>MSTTANKERCLEMVAAWNRWDVSGVVAHWAPDVVHYDDEDKPVSAEEVVRRMNSAVEAFPDLRLDVRSIVGEGDRVMLRITCSATHQGVFMGIAPTGRKVRWTYLEELRFSEAGKVVEHWDVFNFSPLFRDLGVVPDGLKLAAALE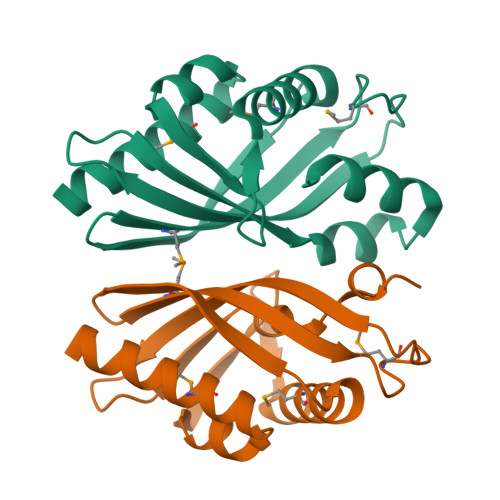HHHHHH[2x]> SLRPKLSEEQQRIIAILLDAHHKTYDPTYSDFCQFRPPVRVNDGGGSVTLELLQLSMLPHLADLVSYSIQKVIGFAKMIPGFRDLTSEDQIVLLKSSAIEVIMLRSNESFTMDDMSWTCGNQDYKYRVSDVTKAGHSLELIEPLIKFQVGLKKLNLHEEEHVLLMAICIVSPDRPGVQDAALIEAIQDRLSNTLQTYIRCRHPPPGSHLLYAKMIQKLADLRSLNEEHSKQYRCLSFQPECSMKLTPLVLEVFGNEG

The vitamin D receptor (VDR), a member of the nuclear receptor (NR) superfamily, orchestrates calcium homeostasis and bone mineralization through transcriptional control of VDR target genes in various tissues. VDR is a ligand-dependent transcription factor that forms an obligate heterodimer with retinoid X receptor α (RXRα). Helices 3, 5, and 12 of the structured LBD serve as the ligand-dependent activation function 2 (AF2) surface for complementary binding of co-regulator proteins (e.g., the p160 family of steroid receptor co-activators such as SRC1). Agonist binding in the hydrophobic pocket of LBD facilitates AF2 to adopt a conformational rearrangement that facilitates high affinity docking of co-regulatory proteins possessing conserved helical nuclear receptor box (NR box) motifs (5′—LXXLL—3′) that dock into the AF2 surface.

Here we present the co-crystal structure of the VDR LBD-VDRM complex at a 2.2 Å resolution. The VDR LBD displays the canonical α-helical sandwich similar to that observed in most NRs, and in this structure Cmpd3 assumes a curve shaped conformation accommodating the hydrophobic ligand binding pocket (LBP). The 5-amino tetrazole amide moiety of Cmpd3 occupies the 1,25D3 A-ring region of the VDR LBP, hydrogen bonding directly with Ser237 (H3) and through water to Tyr143 (H1) and Ser278 (Loop5). The secondary alcohol of Cmpd3 adopts the same bifurcated positioning between His305 (Loop 6) and His397 (H11) as 1,25D3 albeit with a slightly reduced hydrogen bonding distance between both residues and the oxygen atom (2.71 Å vs. 2.81 Å), as shown in Fig. 1c. Consistent with the crystal structure data, peptides that contain these residues all displayed strong protection to solvent exchange in the corresponding HDX studies. All compounds (Cmpd1–3 and 1,25D3) occupy a similar overall orientation and binding location in within the LBD. Despite being a weaker binder, interaction with this non-calcemic ligand afforded a similar extent of protection at VDR H12 compared to that of 1,25D3.> MNARSTGQHPARYPGAAAGEPTLDSWQEPPHNRWAFAHLGEMVPSAAVSRRPVNAPGHALARLG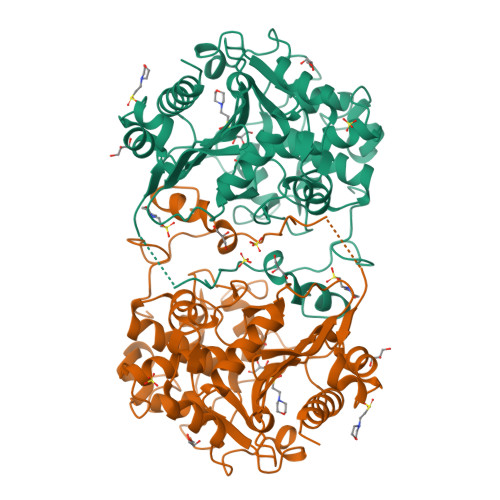AIAAQLPDLEQRLEQTYTDAFLVLRGTEVVAEYYRAGFAPDDRHLLMSVSKSLCGTVVGALVDEGRIDPAQPVTEYVPELAGSVYDGPSVLQVLDMQISIDYNEDYVDPASEVQTHDRSAGWATRRHGDPADTYEFLTTLRGDGSTGEFQYCSANTDVLAWIVERVTGLRYVEALSTYLWAKLDADRDATITVDTTGFGFANGGVSCTARDLARVGRMMLDGGVAPGGRVVSEDWVRRVLAGGSHEAMTDKGFTNTFPDGSYTRQWWCTGNERGNVSGIGIHGQNLWLDPLTDSVIVKLSSWPDPYTEHWHRLQNGILLDVSRALDAV> SASEEQVAQDTEEVFRSYVFYRHQQEQEAEGVAAPADPEMVTLPLQP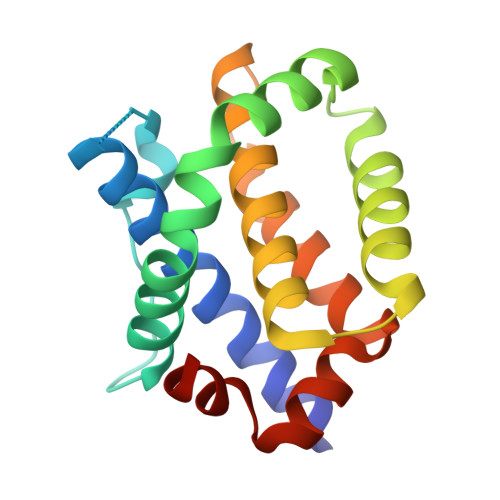SSTMGQVGRQLAIIGDDINRRYDSEFQTMLQHLQPTAENAYEYFTKIATSLFESGINWGRVVALLGFGYRLALHVYQHGLTGFLGQVTRFVVDFMLHHCIARWIAQRGGWVAALNLCNG>[2x]AMSRSRPELGDWSSPAELAELQRSQLPRVLAQALRSPFYAARYRGTTPPRTADDFAGVEVTAKQDLRDQYPFGMLAVGREHLATYHESSGTAGEPTASYYTEEDWTDLAERFARKWTGI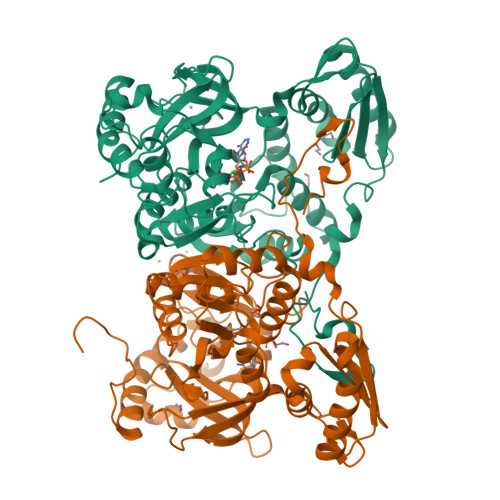HPSDTFLVRTPYGLVITGHLAQAAGRLRGATVVPGDARSLATPLSRMVRVLKTLDVTLTWCNPTEITMLAAAAKAAGLRPDQDFPHLRAMFTAAEPLTEVRRRRLSEIWGGIPVVEEYGSTETGTIAGQCPEGRMHLWADRAIFEVYDPRTGTLSEAGRGQMVVTPLYRDAMPLLRYNLADDVEVSTDPCGCGWLLPTVTVLGRAGTGHRIGPATVTQQRLEELVFSLPAAYEVMFWRAKAHPDVLELEFEAPEPVRQRAVKELGAALDRELGVPHRITGLAPGTLVPAEALTAQRDILKARYLFAEDEDWDKAVMYF> MGHHHHHHGRWAKILEKDKRTQQMRMQRLKAKLQMPFQSGEFKALTRRLQVEPRLLSKQMAGCLEDCTRQAPESPWEEQLARLLQEAPGKLSLDVEQAPSGQHSQAQLSGQQQRLLAFFKCCLLTDQLPLAHHLLVVHHGQRQKRKLLTLDMYNAVMLGWARQGAFKELVYVLFMVKDAGLTPDLLSYAAALQCMGRQDQDAGTIERCLEQMSQEGLKLQALFTAVLLSEEDRATVLKAVHKVKPTFSLPPQLPPPVNTSKLLRDVYAKDGRVSYPKLHLPLKTLQCLFEKQLHMELASRVCVVSVEKPTLPSKEVKHARKTLKTLRDQWEKALCRALRETKNRLEREVYEGRFSLYPFLCLLDEREVVRMLLQVLQALPAQGESFTTLARELSARTFSRHVVQRQRVSGQVQALQNHYRKYLCLLASDAEVPEPCLPRQYWEALGAPEALREQPWPLPVQMELGKLLAEMLVQATQMPCSLDKPHRSSRLVPVLYHVYSFRNVQQIGILKPHPAYVQLLEKAAEPTLTFEAVDVPMLCPPLPWTSPHSGAFLLSPTKLMRTVEGATQHQELLETCPPTALHGALDALTQLGNC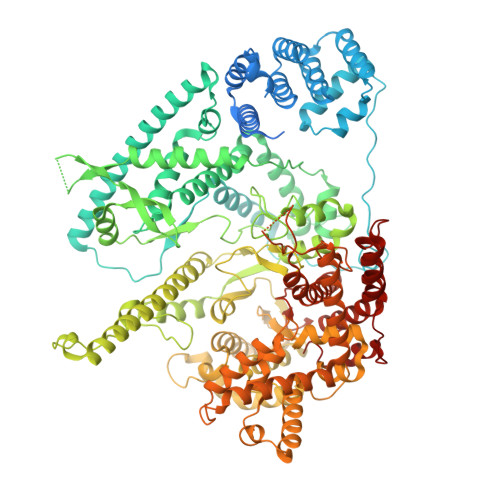AWRVNGRVLDLVLQLFQAKGCPQLGVPAPPSEAPQPPEAHLPHSAAPARKAELRRELAHCQKVAREMHSLRAEALYRLSLAQHLRDRVFWLPHNMDFRGRTYPCPPHFNHLGSDVARALLEFAQGRPLGPHGLDWLKIHLVNLTGLKKREPLRKRLAFAEEVMDDILDSADQPLTGRKWWMGAEEPWQTLACCMEVANAVRASDPAAYVSHLPVHQDGSCNGLQHYAALGRDSVGAASVNLEPSDVPQDVYSGVAAQVEVFRRQDAQRGMRVAQVLEGFITRKVVKQTVMTVVYGVTRYGGRLQIEKRLRELSDFPQEFVWEASHYLVRQVFKSLQEMFSGTRAIQHWLTESARLISHMGSVVEWVTPLGVPVIQPYRLDSKVKQIGGGIQSITYTHNGDISRKPNTRKQKNGFPPNFIHSLDSSHMMLTALHCYRKGLTFVSVHDCYWTHAADVSVMNQVCREQFVRLHSEPILQDLSRFLVKRFCSEPQKILEASQLKETLQAVPKPGAFDLEQVKRSTYFFS> MHKITPFLIAAVVAVIVLAVWLFKKDNKK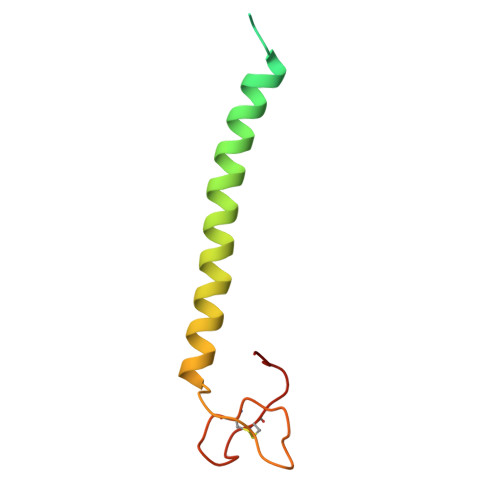ETWFSRDLNYGKANSKIWNATVAKGLKGIANENAEIRKMYPYLGYGDFTGAICKGPNNQGCTYYANYTR>GAMTSQINRQYQLAQRPSGLPGRDTFSFVETPLGEPAEGQILVKNEYLSLDPAMRGWMNDARSYIPPVGIGEVMRALGVGKVLVSKHPGFQAGDYVNGALGVQDYFIGEPKGFYKVDPSRAPLPRYLSALGMTGMTAYFALLDVGQPKNGETVVISGAAGAVGSVAGQIARLKGCRVVGIAGGAEKCRFLVEELG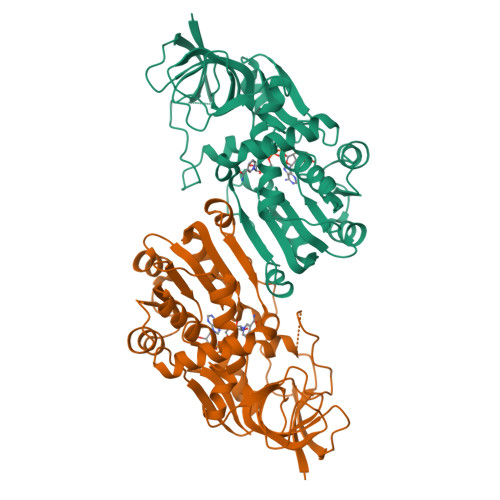FDGAIDYKNEDLAAGLKRECPKGIDVFFDNVGGEILDTVLTRIAFKARIVLCGAISQYNNKEAVRGPANYLSLLVNRARMEGMVVMDYAQRFPEGLKEMATWLAEGKLQSREDIVEGLETFPETLLKLFSGENFGKLVLKV[12x]>[2x]VLGKPQTDPTLEWFLSHCHIHKYPSKSTLIHQGEKAETLYYIVKGSVAVLIKHEEGKEMILSYLNQGDFIGELGLFEEGQERSAW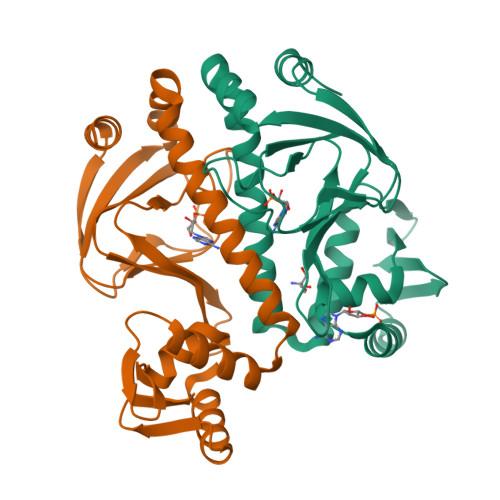VRAKTACEVAEISYKKFRQLIQVNPDILMRLSAQMARRLQVTSEKVGNLAFLDVTGRIAQTLLNLAKQPDAMTHPDGMQIKITRQEIGQIVGCSRETVGRILKMLEDQNLISAHGKTIVVYGTR> GIILQTYRAIADYEKTSGSEMALSTGDVVEVVEKSESGWWFCQMKGKRGWIPASFLEPLDSPDETEDPEPNYAGEPYVAIKAYTAVEGDEVSLLEGEAVEVIHKLLDGWWVIRKDDVTGYFPSMYLQKSGQ;> PP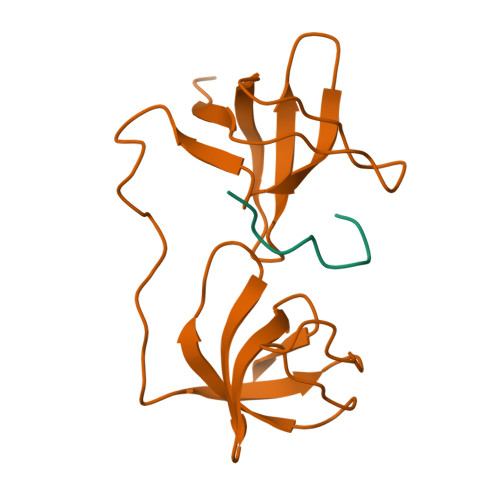SNPPPRPPAEARKKPS2,6-anhydro-3,5-dideoxy-5-[(hydroxyacetyl)amino]-D-glycero-L-altro-non-2-enonic acid | C11 H17 N O9 | 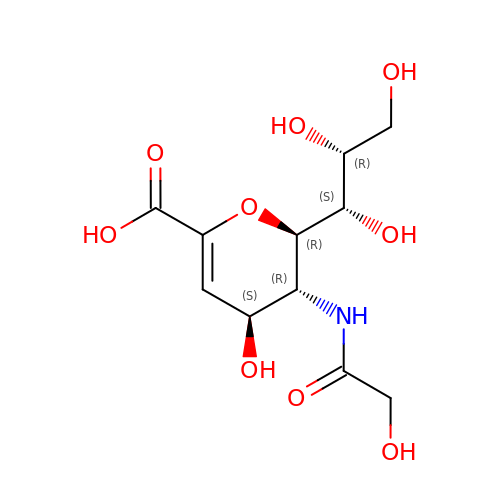FDONZIZJWIPGCO-CYVDNQRASA-N> MSSALTDLFPLPIVQAPMAGGVSVPQLAAAVCEAGGLGFLAAGYKTADGMYQEIKRLRGLTGRPFGVNVFMPQPELAESGAVEVYAHQLAGEAAWYETELGDPDGGRDDGYDAKLAVLLDDPVPVVSFHFGVPDREVIARLRRAGTLTLVTATTPEEARAVEAAGADAVIAQGVEAGGHQGTHRDSSEDDGAGIGLLSLLAQVREAVDIPVVAAGGIMRGGQIAAVLAAGADAAQLGTAFLATDESGAPGPHK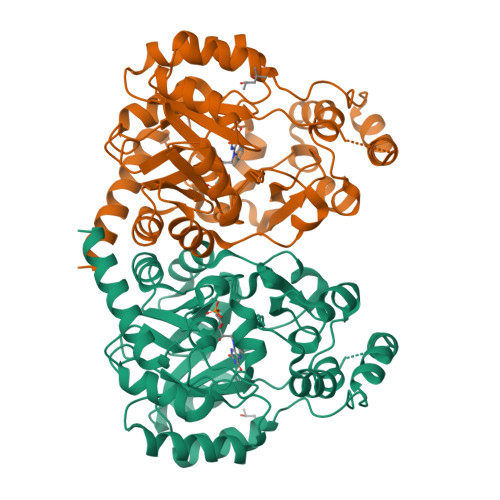RALTDPLFARTRLTRAFTGRPARSLVNRFLREHGPYAPAAYPDVHHLTSPLRKAAAKAGDAQGMALWAGQGHRMARELPAGRLVEVLAAELAEARTALSDASRENESRKGHHHHHH PHENYLMETHYL 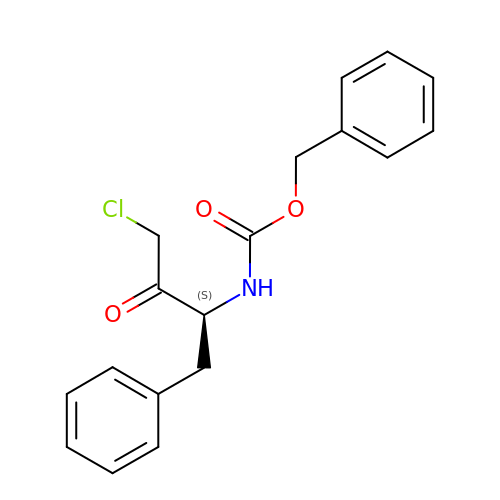N-[(2S)-4-CHLORO-3-OXO-1-PHENYL-BUTAN-2-YL]CARBAMATE | C18 H18 Cl N O3 | OYHLRJGDELITAF-INIZCTEOSA-N3-(2-TERT-BUTYL-5-(PYRIDIN-4-YL)-1H-IMIDAZOL-4-YL)QUINOLINE | C21 H20 N4 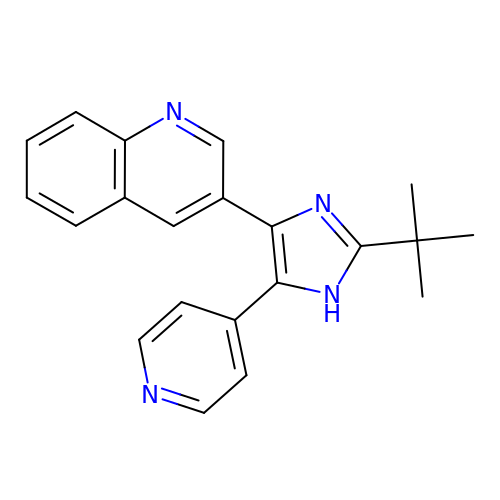| WOMTUQORZZQBPJ-UHFFFAOYSA-N>MKVLEERNAFLSDYEVLKFLTDLEKKHLWDQKSLAALKKSRSKGKQNRPYNHPELQGITRNVVNYLSINKNFINQEDEGEERESSGA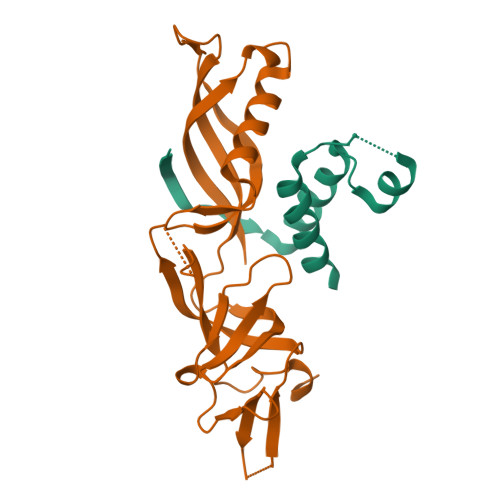KDAEKSGISKMSDESFAELMTKLNSFKLFKAEKLQIVNQLPANMVHLYSIVEECDARFDEKTIEEMLEIISAYA[2x];>[2x]MFILSKIADLVRIPPDQFHRDTISAITHQLNNKFANKIIPNVGLCITIYDLLTVEEGQLKPGDGSSYINVTFRAVVFKPFLGEIVTGWISKCTAEGIKVSLLGIFDDIFIPQNMLFEGCYYTPEESAWIWPMDEETKLYFDVNEKIRFRIEREVFVDVKPKSPKERELEERAQLENEIEGKNEETPQNEKPPAYALLGSCQTDGMGLVSWWEHHHHHH>[6x]SNAMKTVTVRDLVVGEGAPKIIVSLMGKTITDVKSEALAYREADFDILEWRVDHFANVTTAESVLEAAGAIREIITDKPLLFTFRSAKEGGEQALTTGQYIDLNRAAVDSGLVDMIDLELFTGDDEVKATVGYAHQHNVAVIMSNHDFHKTPAAEEIVQRLRKMQELGADIPKIAVMPQTKADVLTLLTATVEMQERYADRPIITMSMSKTGVISRLAGEVFGSAATFGA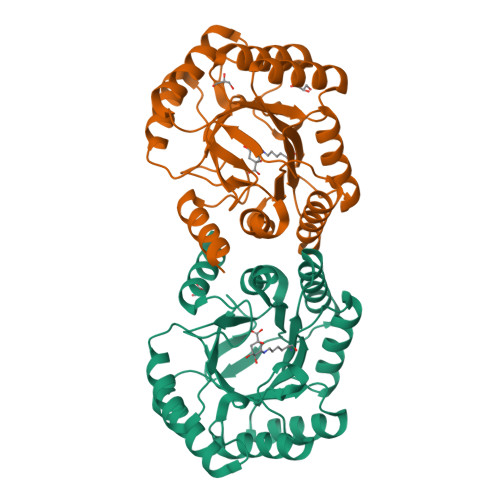VKKASAPGQISVADLRTVLTILHQA>AMSKLNRIRHHLHSVQAELAVFSDPVT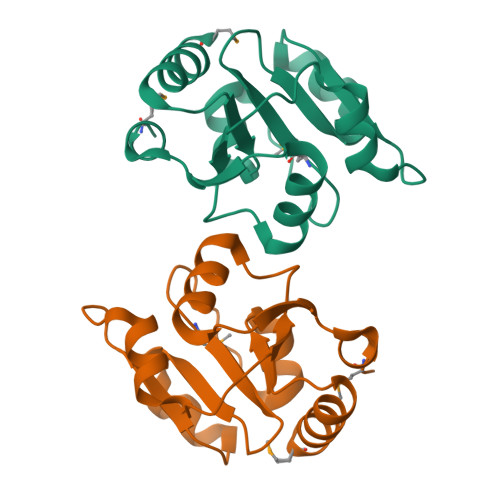VNYLTGFFCDPHERQMFLFVYEDRDPILFVPALEVSRAKQSVPFPVFGYIDSENPWQKIASNLPSFSVSKVLAEFDNLNVTKFQGLQTVFDGHFENLTPYIQNMR[2x]>SQKSWIESTLTKRECVYIIPSSKDPHRCLPGCQICQQLVRCFCGRLVKQHACFTASLAMKYSDVKLGEHFNQAIEEWSVEKHTEQSPTDAYGVINFQGGSHSYRAKYVRLSYDTKPEIILQLLLKEWQMELPKLVISVHGGMQKFELHPRIKQLLGKGLIKAAVTTGAWILTGGVNTGVAKHVGDALKEHASRSSRKICTIGIAPWGVIENRNDLVGRDVVAPYQTLLNPLSKLNVLNNLHSHFILVDDGTVGKYGAEVRLRRELEKTINQQRIHARIGQGVPVVALIFEGGPNVILTVLEYLQESPPVPVVVCEGTGRAADLLAYIHKQTEEGGNLPDAAEPDIISTIKKTFNFGQSEAVHLFQTMMECMKKKELITVFHIGSEDHQDIDVAILTALLKGTNASAFDQLILTLAWDRVDIAKNHVFVYGQQWLVGSLEQAMLDALVMDRVSFVKLLIENGVSMHKFLTIPRLEELYNTKQGPTNPMLFHLIRDVKQGNLPPGYKITLIDIGLVIEYLMGGTYRCTYTRKRFRLIYNSLGGNNRRSGRNTSSSTPQLRKSHETFGNRADKKEKMRHNHFIKTAQPYRPKMDASMEEGKKKRTKDEIVDIDDPETKRFPYPLNELLIWACLMKRQVMARFLWQHGEESMAKALVACKIYRSMAYEAKQSDLVDDTSEELKQYSNDFGQLAVELLEQSFRQDETMAMKLLTYELKNWSNSTCLKLAVSSRLRPFVAHTCTQMLLSDMWMGRLNMRKNSWYKVILSILVPPAILMLEYKTKAEMSHIPQSQDAHQMTMEDSENNFHNITEEIPMEVFKEVKILDSSDGKNEMEIHIKSKKLPITRKFYAFYHAPIVKFWFNTLAYLGFLMLYTFVVLVKMEQLPSVQEWIVIAYIFTYAIEKVREVFMSEAGKISQKIKVWFSDYFNVSDTIAIISFFVGFGLRFGAKWNYINAYDNHVFVAGRLIYCLNIIFWYVRLLDFLAVNQQAGPYVMMIGKMVANMFYIVVIMALVLLSFGVPRKAILYPHEEPSWSLAKDIVFHPYWMIFGEVYAYEIDVCANDSTLPTICGPGTWLTPFLQAVYLFVQYIIMVNLLIAFFNNVYLQVKAISNIVWKYQRYHFIMAYHEKPVLPPPLIILSHIVSLFCCVCKRRKKDKTSDGPKLFLTEEDQKKLHDFEEQCVEMYFDEKDDKFNSGSEERIRVTFERVEQMSIQIKEVGDRVNYIKRSLQSLDSQIGHLQDLSALTVDTLKTLTAQKASEASKVHNEITRELSISKHLAQNLID[4x]

The transient receptor potential channel TRPM7 is a master regulator of the organismal balance of divalent cations that plays an essential role in embryonic development, immune responses, cell mobility, proliferation, and differentiation. TRPM7 represents a master regulator of the cellular balance of divalent cations and mediates uptake of Zn2+, Mg2+ and Ca2+, which is required for the normal prenatal development and healthy adulthood. The TRPM7 structure represents a tetramer assembled of four identical subunits, with the overall architecture reminiscent of other TRPM channels. Each TRPM7 subunit consists of an intracellular N-terminal domain (NTD, residues 1–789), transmembrane domain (TMD, 839–1146), and cytosolic C-terminal domain (CTD, 1157–1230).

First, we determined structures of TRPM7 in the apo state by subjecting the protein purified in glyco-diosgenin (GDN) detergent or reconstituted in lipid nanodiscs to cryo-EM. The corresponding 3D reconstructions resulted in 2.61-Å and 2.19-Å resolution structures. Despite the two structures being nearly indistinguishable, the cryo-EM map for the protein reconstituted in lipid nanodiscs had better overall quality and resolution than the one for the protein purified in GDN. Since all previously published TRPM7 structures represented a single closed state, the nearly perfect superposition of their resolved regions with the corresponding regions in our structures suggests that our apo-state structures also represent the same closed state, TRPM7Closed. We observed excellent protein density in the TMD surrounded by additional density, which allowed us to build models for 18 lipids per TRPM7Closed subunit. Most of these densities have a head-and-two-tails appearance and most likely represent phospholipids. However, two types of putative lipid densities had a shape drastically different from phospholipids, and we modeled them as cholesterol and GDN. Since we did not introduce cholesterol during protein purification, the corresponding densities in our structure most probably represent endogenous cholesterol molecules that interact with the channel in physiological conditions. On the other hand, GDN was used during the extraction step of purification and likely remains attached to the protein despite the following GDN-free reconstitution into lipid nanodiscs. Finally, we inspected TRPM7Closed and found that the vanilloid-like site in this apo-state structure is occupied by an acyl tail of a lipid molecule that protrudes from the base of the S1–S4 bundle.> MDKAELQKTLQANKIQGNIVSSSDLGSGLSMVIVEVNNQQAPFLATDDGKMIFQAEVLIAQDKSTESRVQEFYKNLYEKEKLRISAKLKEVFKAQKANVFTFKAKKPS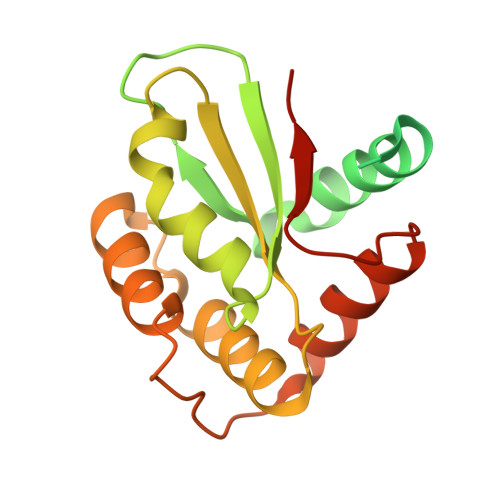NKTIYIVSDFNCPYCQREFANLDKRLESANVELLVVGFLGEDSILKAANALKNKSGNQAKDIAMLQKLYTPKSKGQSMDIKAAMALTQAVADTGVRSVPYIIEPHHHHHH> RQLVFLEWHEAPTIAVALLAALGFLSTLAILVIFWRHFQTPIVRSAGGPMCFLMLTLLLVAYMVVPVYVGPPKVSTCLCRQALFPLCFTICISCIAVRSFQIVCAFKMASRFPRAYSYWVRYQGPYVSMAFITVLKMVIVVIGMLATGLSPTTRTDPDDPKITIVSCNPNYRNSLLFNTSLDLLLSVVGFSFAYMGKELPTNYNEAKFITLSMTFYFTSSVSLCTFMSAYSGVLVTIVDLLVTVLNLLAISLGYFGPKCYMILFYPERNTPAYFNSMI;> PRRPKFLAWGEPVVLSLLLLLCLVLGLALAALGLSVHHWDSPLVQASGGSQFCFGLICLGLFCLSVLLFPGRPSSASCLAQQPMAHLPLTGCLSTLFLQAAETFVESELPLSWANWLCSYLRGLWAWLVVLLATFVEAALCAWYLIAFPPEVVTDWSVLPTEVLEHCHVRSWVSLGLVHITNAMLAFLCFLGTFLVQSQPGRYNRARGLTFAMLAYFITWVSFVPLLANVQVAYQPAVQMGAILVCALGILVTFHLPKCYVLLWLPKLNTQEFFL

Sugars and other sweet-tasting compounds are detected by the sweet taste receptor, a member of the class C GPCR family. The sweet receptor is a heterodimer composed of TAS1R2 and TAS1R3,3,4 two type 1 taste receptor family members that share the distinctive architecture of class C GPCRs: a large extracellular Venus flytrap (VFT) domain, responsible for ligand recognition; a cysteine-rich domain (CRD); and a seven-transmembrane (7TM) domain that mediates G protein coupling. To address this gap, here we present cryo-electron microscopy (cryo-EM) structures of the sweet receptor in the inactive, unliganded state, as well as in the activated, sucralose- and advantame-bound states. Unlike other class C GPCRs, such as mGluR, CaSR and GABAB receptors, where agonists stabilize inter-subunit VFT interactions to promote activation, the sweet receptor is activated by the rearrangement of a TAS1R2 VFT loop, which destabilizes interactions between the lower VFT lobes and the VFT–CRD interfaces.

We first determined the structure of the human/mouse sweet receptor in the absence of sweeteners. To improve the resolution, we combined all particles to generate a global reconstruction at 3.1 Å resolution, then performed local refinement focused on the VFT/CRD region or the 7TM domain, obtaining final resolutions of 2.9 Å and 3.6 Å, respectively. While the orientation between extracellular and transmembrane domains can vary, each domain remains nearly identical across individual classes. In our apo sweet receptor structure, the two subunits pack closely against each other at both the upper and lower lobes of the VFT domains, as well as at the 7TM domains. In the apo state, the 7TM domains of TAS1R2 and TAS1R3 interact through two interfaces, a configuration that is markedly different from that seen in other apo-state class C GPCRs.> GPGSLGSGAYRSVGEWLEAIKMGRY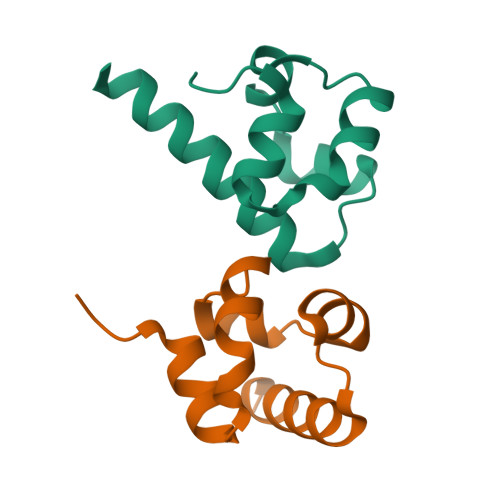TEIFMENGYSSMDAVAQVTLEDLRRLGVTLVGHQKKIMSSLQEMKVQMVNGMVPV;> GPGSMCTNIVYEWLKALQLPQYAESFVDNGYDDLEVCKQIGDPDLDAIGVLAPAHRRRILEAVHRLREQD>GPLGSAYQLLLSKETLNKILQYKQNLEKGLATPGKFFLEELSKQEKSISEMDITTFTQLLIQSKKPQVFAESQVYHDGTDWTLEEESILGDVSVNMPVTMYNDGGHGSSFKNHPKPISGYLAYVPGALLASGSGPTSDMKEVLDNGKLNQDKLNALYERRLLPQLIHFNELARQNEKQAAITIPGIGTGCFSGAYYDVIKPYVRNALIHILEKHKDSLPYIDIIHYDPYMGDEPAEKKIGHMSFRVSPSGVVRGTTGQLDYPLGSNPDTHILVSIVAWDHFSWPGNDYWGGARQTDDGVKAASTDTMGQVTGATGVYDKKWGRYMPPE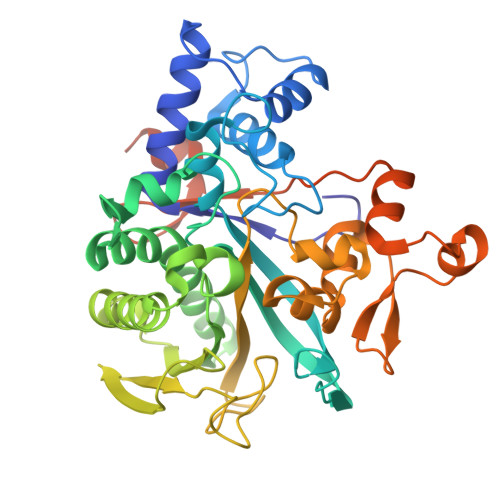SFTKDRKGMSDWGDYVRENGIVFNGPVLALDKSGKLDTLENVASRSSKAKVETTTTISDLVRSMFSLFSHS[8x]> ANPEQLKHCNGILKELLSKKHAAYAWPFYKPVDASALGLH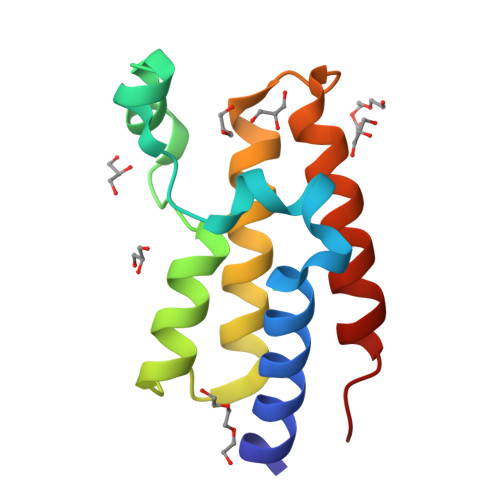DYHDIIKHPMDLSTVKRKMENRDYRDAQEFAADVRLMFSNCYKYNPPDHDVVAMARKLQDVFEFRYAKMPD>[2x]MEKKTIVLGVIGSDCHAVGNKILDHAFTNAGFNVVNIGVLSPQENFIKAAIETKADAILVSSLYGQGEIDCKGLRQKCDEAGLEGILLYVGGNIVVGKQHWPDVEKRFKDMGYDRVYAPGTPPEVGIADLKKDLNIE;>MELKNKKWTDEEFHKQREEVLQQWPTGKEVDLQEAVDYLKKIPAEKNFAEKLVLAKKKGITMAQPRAGVALLDEHIELLRYLQDEGGADFLPSTIDA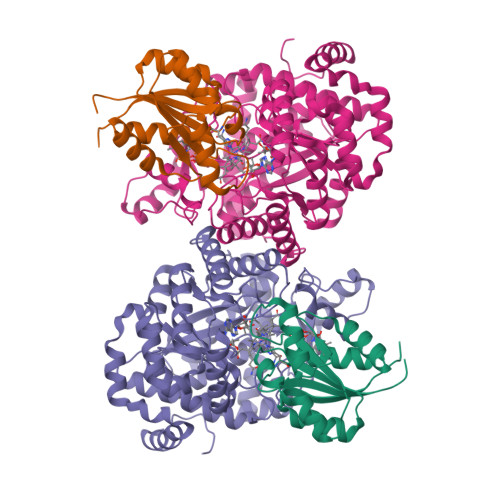YTRQNRYDECENGIKESEKAGRSLLNGFPGVNFGVKGCRKVLEAVNLPLQARHGTPDSRLLAEIIHAGGWTSNEGGGISYNVPYAKNVTIEKSLLDWQYCDRLVGFYEEQGVHINREPFGPLTGTLVPPSMSNAVGITEALLAAEQGVKNITVGYGECGNMIQDIAALRCLEEQTNEYLKAYGYNDVFVTTVFHQWMGGFPQDESKAFGVIVTATTIAALAGATKVIVKTPHEAIGIPTKEANAAGIKATKMALNMLEGQRMPMSKELETEMAVIKAETKCILDKMFELGKGDLAIGTVKAFETGVMDIPFGPSKYNAGKMMPVRDNLGCVRYLEFGNVPFTEEIKNYNRERLQERAKFEGRDVSFQMVIDDIFAVGKGRLIGRPE[2x]>[2x]MPISPIETVPVKLKPGMDGPKVKQWPLTEEKIKALVEICTEMEKEGKISKIGPENPYNTPVFAIKKKDSTKWRKLVDFRELNKRTQDFWEVQLGIPHPAGLKKKKSVTVLDVGDAYFSVPLDEDFRKYTAFTIPSINNETPGIRYQYNVLPQGWKGSPAIFQSSMTKILEPFRKQNPDIVIYQYMDDLYVGSDLEIGQHRTKIEELRQHLLRWGLTTPDKKHQKEPPFLWMGYELHPDKWTVQPI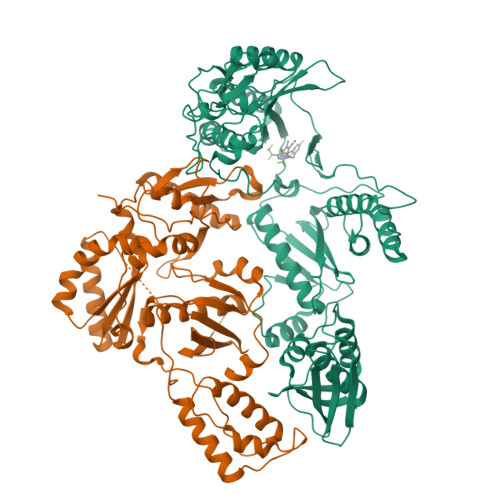VLPEKDSWTVNDIQKLVGKLNWASQIYPGIKVRQLCKLLRGTKALTEVIPLTEEAELELAENREILKEPVHGVYYDPSKDLIAEIQKQGQGQWTYQIYQEPFKNLKTGKYARMRGAHTNDVKQLTEAVQKITTESIVIWGKTPKFKLPIQKETWETWWTEYWQATWIPEWEFVNTPPLVKLWYQLEKEPIVGAETFYVDGAANRETKLGKAGYVTNRGRQKVVTLTDTTNQKTELQAIYLALQDSGLEVNIVTDSQYALGIIQAQPDQSESELVNQIIEQLIKKEKVYLAWVPAHKGIGGNEQVDKLVSAGIRKVL> MGSSHHHHHHSSENLYFQGHMKAEVSQQRSLLTLSEVDAELARIAHRGKNLAEQKRLDELTAQRGEVNDRLAALGIALEDLDAQVAKYESEIDSVRQREDRDRALLEGGSVGAKQVTEIQHELETLQRRQASLEEQLLEVMERREELMAERSEELRRVDELQTELTEAQQARDAALVELDQARHQCATRRDALVNAIDDQLVELYEKQRARGGAGAGPLQGRRCGACRIEIDRGEIARITAAADDDVVRCPECGAILLRVKQ

The MSMEG_4306 gene in Mycobacterium smegmatis encodes a protein of unknown function, and its homologue Rv2229c in M. tuberculosis has been shown to be essential for survival. Amino-acid sequence analysis of MSMEG_4306 does not indicate statistically significant similarity to any protein of known function. The crystal structure of MSMEG_4306 reveals a long coiled-coil helical domain in its N-terminal region and a zinc-ribbon domain in its C-terminal region. However, considering the near-identical domain organization in both HP0958 and CT398 to that of MSMEG_4306 and the near-identical function of HP0958 and CT398 despite low sequence identity (26%), we predict that MSMEG_4306 might be involved in secretion systems, possibly interacting with multiple entities (proteins or nucleic acids).

Since the two homologues are likely to be too distantly related for successful molecular replacement, we decided to solve the structure of MSMEG_4306 by experimental phasing. Taking advantage of the presence of zinc ion in the MSMEG_4306 crystal, as confirmed by an X-ray fluorescence scan, an X-ray diffraction data set was collected at a wavelength corresponding to the Zn K edge using synchrotron radiation. Here, we report the crystal structure of MSMEG_4306 initially determined by zinc SAD phasing at 2.8 Å resolution and subsequently extended to 2.6 Å resolution. The structure of MSMEG_4306 was solved by zinc SAD phasing using the CRANK2 pipeline as implemented in CCP4. CRANK2 was able to locate one zinc ion and built a partial model for MSMEG_4306 with five fragments totalling 227 residues and identified the space group as P3121. The partial model thus obtained was further refined using REFMAC5 and phenix.refine, and the model was built manually using Coot. By assuming the presence of one molecule in the asymmetric unit, the crystal had a Matthews coefficient of 2.72 Å3 Da−1 with a solvent content of 55%.>MKLYVFLVNTGTTLTFDTELTVQTVADLKHAIQSKYKIAIQHQVLVVNGGECMAADRRVCTYSAGTDTNPIFLFNKEMILCDRPPAIPKTTFSTENDMEIKVEESLMMPAVFHTVASRTQLALEMYEVAKKLCSFCEGLVHDEHLQHQGWAAI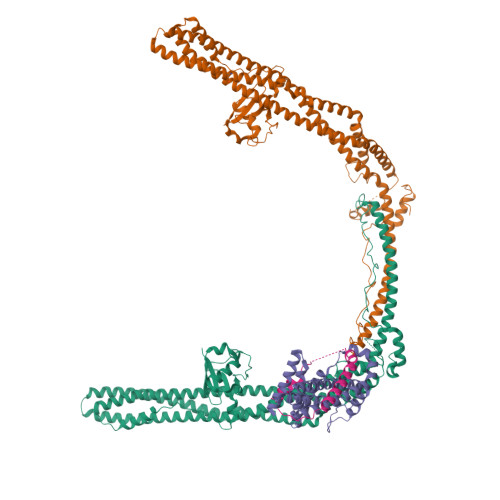MANLEDCSNSYQKLLFKFESIYSNYLQSIEDIKLKLTHLGTAVSVMAKIPLLECLTRHSYRECLGRLDSLPEHEDSEKAEMKRSTELVLSPDMPRTTNESLLTSFPKSVEHVSPDTADAESGKEIRESCQSTVHQQDETTIDTKDGDLPFFNVSLLDWINVQDRPNDVESLVRKCFDSMSRLDPRIIRPFIAECRQTIAKLDNQNMKAIKGLEDRLYALDQMIASCGRLVNEQKELAQGFLANQKRAENLKDASVLPDLCLSHANQLMIMLQNHRKLLDIKQKCTTAKQELANNLHVRLKWCCFVMLHADQDGEKLQALLRLVIELLERVKIVEALSTVPQMYCLAVVEVVRRKMFIKHYREWAGALVKDGKRLYEAEKSKRESFGKLFRKSFLRNRLFRGLDSWPPSFCTQKPRKFDCELPDISLKDLQFLQSFCPSEVQPFLRVP[2x];> HTEILRGLRFTLLFVQHVLEIAALKGSASEAAGGPEYQLQESVVADQISLLSREWGFAEQLVLYLKVAELLSSGLQSAIDQIRAGKLCLSSTVKQVVRRLNELYKASVVSCQGLSLRLQRFFLDKQRLLDRIHSITAERLIFSHAVQMVQSAALDEMFQHREGCVPRYHKALLLLEGLQHMLSDQADIENVTKCKLCIERRLSAL;> DLGTFYREFQNPPQLSSLSIDIGAQSMAEDLDSLPEKLAVHEKNVREFDAFVETLQGSDEA>[2x]GSMAKPLTDQEKRRQISIRGIVGVENVAELKKSFNRHLHFTLVKDRNVATTRDYYFALAHTVRDHLVGRWIRTQQHYYDKCPKRVYYLSLEFYMGRTLQNTMINLGLQNACDEAIYQLGLDIEELEEIEEDAGLGNGGLGRLAACFLDSMATLGLAAYGYGIRYEYGIFNQKIRDGWQVEEADDWLRYGNPWEKSRPEFMLPVHFYGKVEHTNTGTK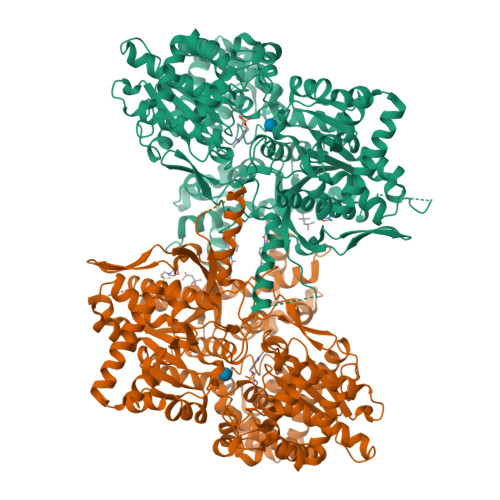WIDTQVVLALPYDTPVPGYMNNTVNTMRLWSARAPNDFNLRDFNVGDYIQAVLDRNLAENISRVLYPNDNFFEGKELRLKQEYFVVAATLQDIIRRFKASKFGSTRGAGTVFDAFPDQVAIQLNDTHPALAIPELMRIFVDIEKLPWSKAWELTQKTFAYTNHTVLPEALERWPVDLVEKLLPRHLEIIYEINQKHLDRIVALFPKDVDRLRRMSLIEEEGSKRINMAHLCIVGSHAVNGVAKIHSDIVKTKVFKDFSELEPDKFQNKTNGITPRRWLLLCNPGLAELIAEKIGEDYVKDLSQLTKLHSFLGDDVFLRELAKVKQENKLKFSQFLETEYKVKINPSSMFDVQVKRIHEYKRQLLNCLHVITMYNRIKKDPKKLFVPRTVIIGGKAAPGYHMAKMIIKLITSVADVVNNDPMVGSKLKVIFLENYRVSLAEKVIPATDLSEQISTAGTEASGTGNMKFMLNGALTIGTMDGANVEMAEEAGEENLFIFGMRIDDVAALDKKGYEAKEYYEALPELKLVIDQIDNGFFSPKQPDLFKDIINMLFYHDRFKVFADYEAYVKCQDKVSQLYMNPKAWNTMVLKNIAASGKFSSDRTIKEYAQNIWNVEPSDLKISLSNESNKVNGN>MTTNLTNSNCVEEYKENGKTKIRIKPFNALIELYHHQTPTGSIKENLDKLENYVKDVVKAKGLAIPTSGAFSNTRGTWFEVMIAIQSWNYRVKRELNDYLIIKMPNVKTFDFRKIFDNETREKLHQLEKSLLTHKQQVRLITSNPDLLIIRQKDLIKSEYNLP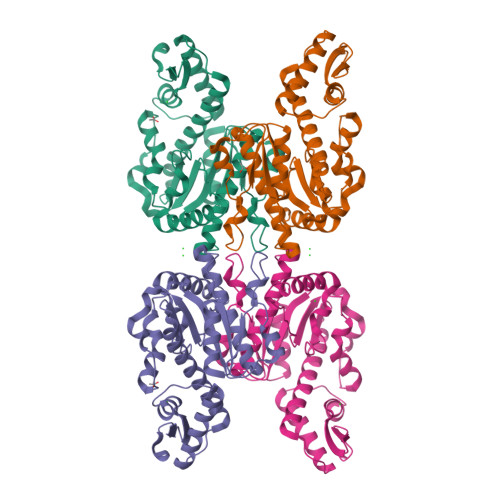INKLTHENIDVALTLFKDIEGKCKWDSLVAGVGLKTSLRPDRRLQLVHEGNILKSLFAHLKMRYWNPKAEFKYYGASSEPVSKADDDALQTAATHTIVNVNSTPERAVDDIFSLTSFEDIDKMLDQIIKK[2x]> MKIAFIGEAVSGFGGMETVISNVIHTFENSSPKINCEMFFFCRNDKMDKAWLKEIKYAQSFSNIKLSFLRRAKHVYNFSQWLKETSPDIVICIDVISCLYANKARKKSGKHFTIFSWPHFSLDHKKHAECITYADYHLAISSGIKEQIMARGISAQDISVVYNPVSIKTVIVPPPERDKPAVFLYVGRLKFEGQKRVKDLFDGLARTTGEWQLHIIGDGSDFEKCQAYSRELGIEQRV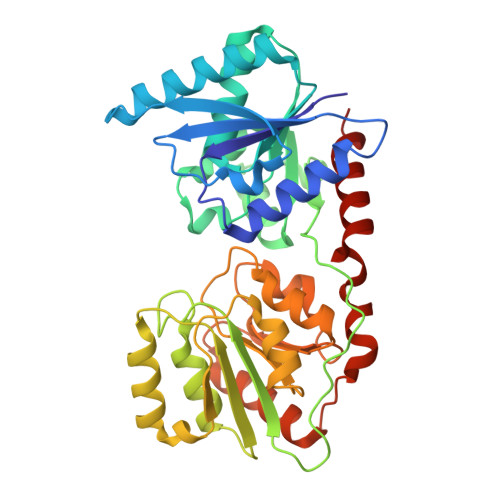IWYGWQSAPWQVVQQKIKNVTALLLTSAFEGFPMTLLEAMSYGIPCISSDCMSGPRDMIKPGLNGELYTPGAIDDFVGHLNRVISGEVKYQHDIIPGTIERFYDVLYFKNFNNAIFSKLQK> SSRESMQTIPHYLQ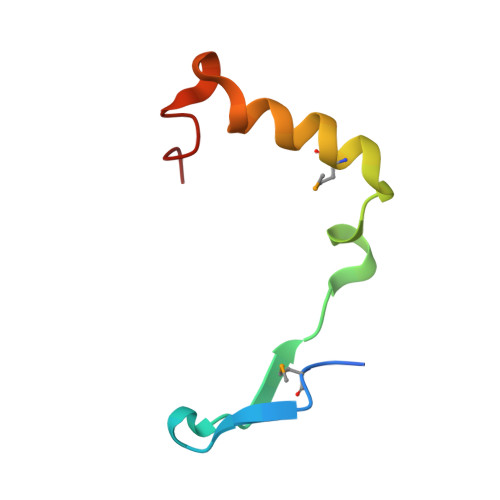IKEILQISKQELLPCHVMEQHWKFYVGRSHSEALLSW> HNELIHDAVLDYYGKRLATCSSDKTIKIFEVEGETHKLIDTLTGHEGPVWRVDWAHPKFGTILASCSYDGKVLIWKEENGRWSQIAVHAVHSASVNS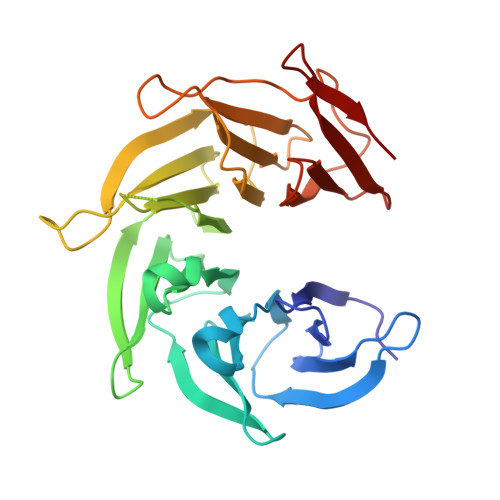VQWAPHEYGPLLLVASSDGKVSVVEFKENGTTSPIIIDAHAIGVNSASWAPATIEEDGEHNGTKESRKFVTGGADNLVKIWKYNSDAQTYVLESTLEGHSDWVRDVAWSPTVLLRSYLASVSQDRTCIIWTQDNEQGPWKKTLLKEEKFPDVLWRASWSLSGNVLALSGGDNKVTLWKENLEGKWEPAG>MNHSDTLSLSLELLQQPSVTPIDHTCQTIMADRLAKVGFHIEPMRFGDVDNLWARRGTEGPVFCFAGHTDVVPTGRLDAWNSDPFAPEIRDGKLYGRGSADMKTALAAMVVASERFVAKHPNHKGSIAFLITSDEEGPAVNGTVKVIETLEKRNEKITWCLVGEPSSTHKLGDIVKNGRRGSLNAVLKVQGKQGHVAYPHLARNPIHEASPALAELCQTVWDNGNEYFPATSFQISNIHAGTGATNVIPGALEVTFNFRYSTEVTAEQLKQRVHEILDKHGLQYEIVWNLSGLPFLTPVGELVNAAQTAILN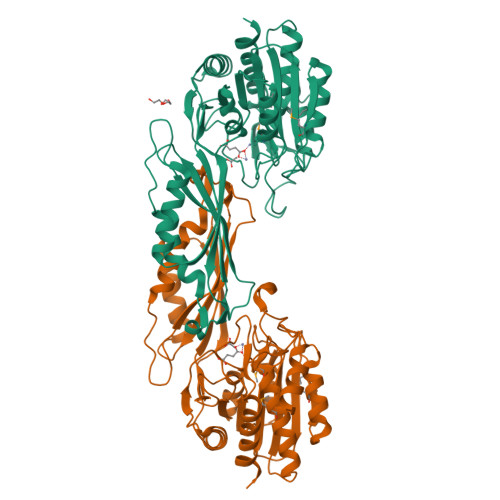VTGTETELSTSGGTSDGRFIAPTGAQVLELGVLNATIHQINEHVDVHDLDPLTDIYEQILENLLAQ[2x]We find that reconstituting the pentameric ligand-gated ion channel (pLGIC), Erwinia ligand-gated ion channel (ELIC), in different nanodiscs produces distinct structures by cryo-EM. ELIC is one of a few pLGICs for which there is an activated, open-channel structure, and is therefore a useful structural model. Activation and opening of the channel involves a tilting of the top of M2 away from the pore axis and partial loss of the helix, such that 16′ and 9′ turn away from the pore. In the extracellular domain (ECD), ELIC activation is characterized by a counter-clockwise rotation of the ECD relative to the TMD.

Single particle cryo-EM of ELIC in these nanodiscs in the presence of the agonist, propylamine (50 mM), yielded structures with an overall resolution of 3.71 Å for SMA, 3.28 Å for saposin, 3.12 Å for spMSP1D1, and 3.17 Å for spNW15. The effective diameter of ELIC, which depends partially on nanodisc size, agrees with the trend observed in the structures except spNW15ELIC. spNW15ELIC produced the largest nanodisc particle as expected for this circularized scaffold which forms 15 nm empty nanodiscs. Comparison of the agonist-bound structures of ELIC in the different nanodiscs also shows progressive tilting of the top of M2 away from the pore axis in the order: SMAELIC < saposinELIC~MSP1E3D1ELIC~spMSP1D1ELIC < spNW15ELIC. This is evident in the mean distance between M2 Cα atoms and the pore axis, especially residues 249–251. spNW15ELIC also shows a significant tilting of the bottom of M2 towards the pore axis and the adjacent subunit, narrowing the pore at 2′ (Q233) and -2′ (E230). However, in spNW15ELIC and all other agonist-bound WT structures, the position of 9′ is unchanged forming a tight constriction of the ion permeation pathway. This is not unlike the desensitized structure of α7 nAchR where 9’ appears to form the desensitization gate; therefore, we suggest that spNW15ELIC is a plausible desensitized structure of ELIC. There is no density for M4 in spNW15ELIC indicating that this helix is structurally heterogeneous in the spNW15 nanodisc. The pore of spNW15ELIC shows widening at the top and narrowing at the bottom to a greater extent than any other WT agonist-bound structure. SMAELIC and spNW15ELIC show the least and greatest agonist-dependent changes, respectively. The nanodisc density for spNW15ELIC was smaller than expected possibly because the position of ELIC within the nanodisc is more heterogeneous.

>APADNAADARPVDVSVSIFINKIYGVNTLEQTYKVDGYIVAQWTGKPRKTPGDKPLIVENTQIERWINNGLWVPALEFINVVGSPDTGNKRLMLFPDGRVIYNARFLGSFSNDMDFRLFPFDRQQFVLELEPFSYNNQQLRFSDIQVYTENIDNEEIDEWWIRGKASTHISDIRYDHLSSVQPNQNEFSRITVRIDAVRNPSYYLWSFILPLGLIIAASWSVFWLESFSERLQTSFTLMLTVVAYAFYTSNILPRLPYTTVIDQMIIAGYGSIFAAILLIIFAHHRQANGVEDDLLIQRCRLAFPLGFLAIGCVLVIRGITL[5x]> MAASQQQASAASSAAGVSGPSSAGGPGPQQQPQPPAQLVGPAQSGLLQQQQQDFDPVQRYKMLIPQLKESLQTLMKVAAQNLIQNTNIDNGQKSSDGPIQRFDKCLEEFYALCDQLELCLRLAHEC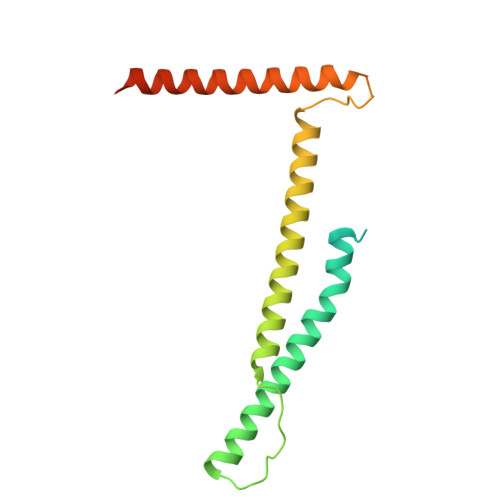LSQSCDSAKHSPTLVPTATKPDAVQPDSLPYPQYLAVIKAQISCAKDIHTALLDCANKVTGKTPAPPAGPGGTL>[2x]TTNKPIVLSTWNFGLHANVEAWKVLSKGGKALDAVEKGVRLVEDDPTERSVGYGGRPDRDGRVTLDACIMDENYNIGSVACMEHIKNPISVARAVMEKTPHVMLVGDGALEFALSQGFKKENLLTAESEKEWKEWLKTSQYKPIVNIENHD;>TIGMIALDAQGNLSGACTTSGMAYKMHGRVGDSPIIGAGLFVDNEIGAATATGHGEEVIRTVGTHLVVELMN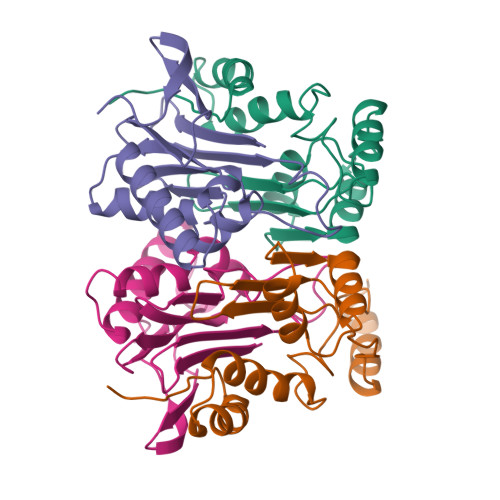QGRTPQQACKEAVERIVKIVNRRGKNLKDIQVGFIALNKKGEYGAYCIQDGFNFAVHDQKGNRLETPGFALK[2x]> MPTRKSNTYLSLVNSYLIDSPQPSSINYWWNLGSLLGLCLVIQIASGVFLAMHYSSNIELAFDSVEHIMRDVNAGWLIRYIHANGASFFFICMYLHIGKALYYGSYKQPRVMLWVIGVVIFILTMAIAFMGYCLVYGQMSHWGATVITNLLSAIPFIGNDIVPFIWGGFSVSNPTIQRFFALHFLLPFILAALVCMHLMALHVHGSSNPVGITGNIDRLPMHPYFIFKDLITVFVFLLIFSLF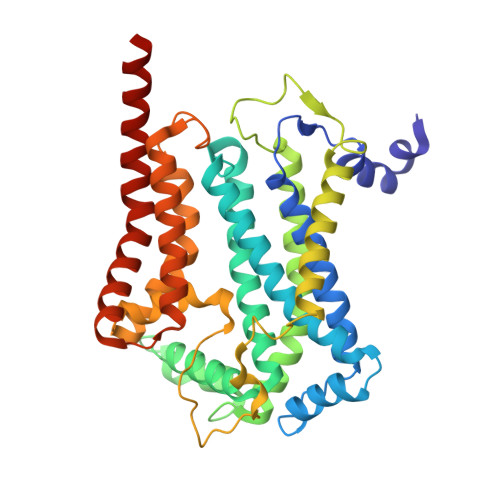VFYSPNTLGHPDNYIPGNPMVTPPSIVPEWYLLPFYAILRSIPDKLGGVIAMFGAILILLSLPYTDRSIIRGNSFKVLSKLAFYLFVFNFILLGNLGQLHVEVPYIQLGQFATAYYFAHYIIVVPVISTLENILYYIGTQTRVK> SDMPVERILEAELAVEPKTETYVEANMGLNPSSPNDPVTNICQAADKQLFTLVEWAKRIPHFSELPLDDQVILLRAGWNELLIASFSHRSIAVKDGILLATGLHVHRNSAHSAGVGAIFDRVLTELVSKMRDMQMD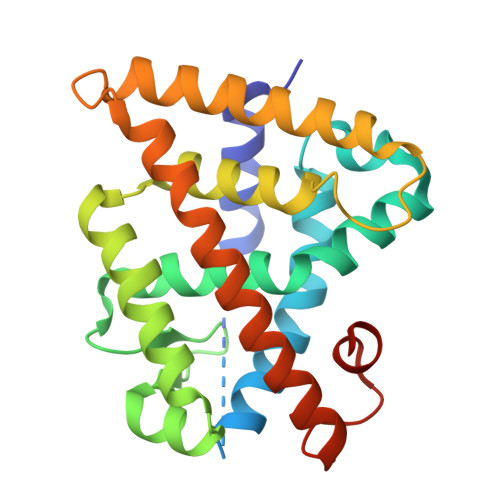KTELGCLRAIVLFNPDSKGLSNPAEVEALREKVYASLEAYCKHKYPEQPGRFAKLLLRLPALRSIGLKCLEHLFFFKLIGDTPIDTFLMEMLEAPHQMT> MADVVVGIQWGDEGKGKIVDRIAKDYDFVVRYQGGHNAGHTIVHKGVKHSLHLMPSGVLYPKCKNIISSAVVVSVKDLCEEISAFEDLENRLFVSDRAHVILPYHAKKDAFKEKSQNIGTTKKGIGPCYEDKMARSGIRMGDLLDDKILEEKLNAHFKAIEPFKKAYDLGENYEKDLMGYFKTYAPKICPFIKDTTSMLIEANQKGEKILLEGAQGTLLDIDLGTYPFVTSSNTTSA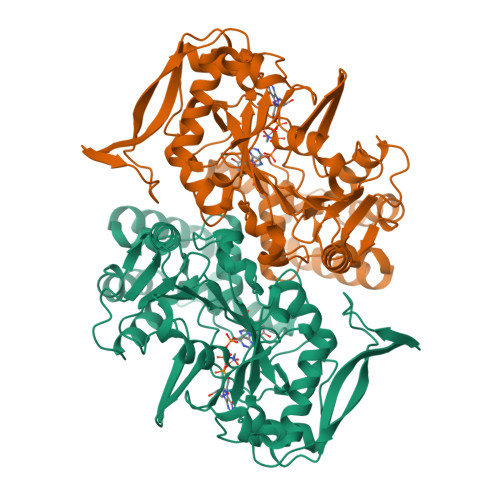SACVSTGLNPKAINEVIGITKAYSTRVGNGPFPSEDTTPMGDHLRTKGAEFGTTTKRPRRCGWLDLVALKYACALNGCTQLALMKLDVLDGIDAIKVCVAYERKGERLEIFPSDLKDCVPIYQTFKGWEKSVGVRKLDDLEPNVREYIRFIEKEVGVKIRLISTSPEREDTIFLLEHHHHHH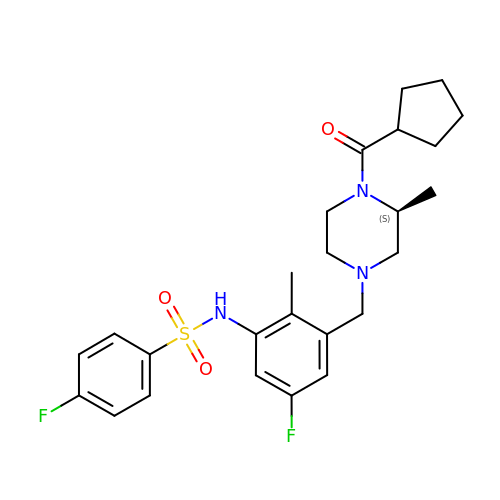N-(3-{[(3S)-4-(cyclopentanecarbonyl)-3-methylpiperazin-1-yl]methyl}-5-fluoro-2-methylphenyl)-4-fluorobenzene-1-sulfonamide | C25 H31 F2 N3 O3 S | BARSGQAUTAPATR-KRWDZBQOSA-N> NSSPSPVPGSQNVPAPAVKKISQYACQRRTTLNNYNQLFTDALDILAENDELRENEGSCLAFMRASSVLKSLPFPITSMKDTEGIPCLGDKVKSIIEGIIEDGESSEAKAVLNDERYKSFKLFTSVFGVGLKTAEKWFRMGFR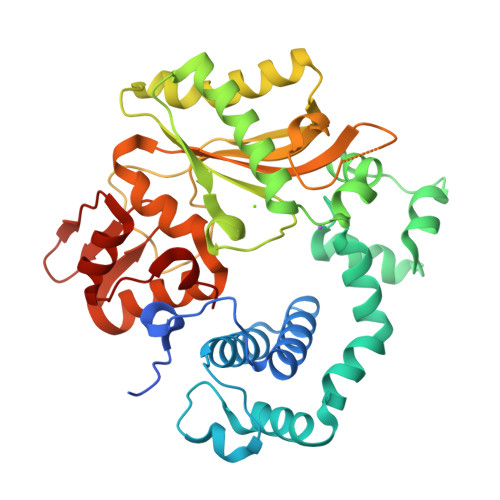TLSKIQSDKSLRFTQMQKAGFLYYEDLVSCVNRPEAEAVSMLVKEAVVTFLPDALVTMTGGFRRGKMTGHDVDFLITSPEATEDEEQQLLHKVTDFWKQQGLLLYCDILESTFEKFKQPSRKVDALDHFQKCFLILKLDHGRVHSEKSGQQEGKGWKAIRVDLVMCPYDRRAFALLGWTGSRQFERDLRRYATHERKMMLDNHALYDRTKRVFLEAESEEEIFAHLGLDYIEPWERNA> GPLGSPEFENKIEDIGQGAEIIKRTQDITSKRLAICQNIQFDFVKDKKYNKDALVVKMQGFISSRTTYSDLKKYPYIKRMIWPFQYNISLKTKDSNVDLINYLPKNKIDSADVSQKLGYNIGGNFQSAPSIGGSGSFNYSKTISYNQKNYVTEVESQNSKGVKWGVKANSFVTPNGQVSAYDQYLFAQDPTGPA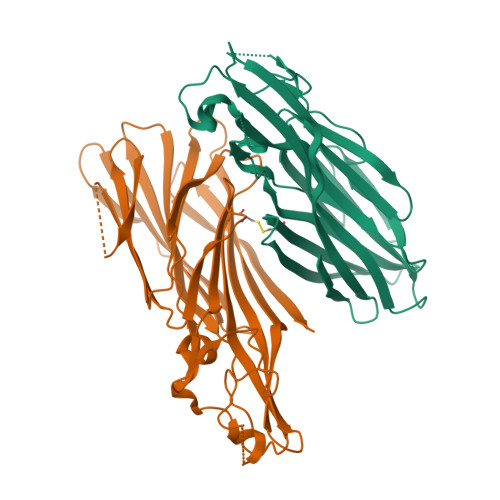ARDYFVPDNQLPPLIQSGFNPSFITTLSHEKGKGDKSEFEITYGRNMDATYAYVTRHRLAVDRKHDAFKNRNVTVKYEVNWKTHEVKIKSITPK;> GPLGSPEFEGKITPVSVKKVDDKVTLYKTTATADSDKFKISQILTFNFIKDKSYDKDTLVLKAAGNINSGYEKPNPNDYDFSKLYWGAKYNVSISSQSNDSVNVVDYAPKNQNEEFQVQNTLGYTFGGDISISNGLSGGLNGNTAFSETINYKQESYRTTLSRCTNYKNVGWGVEAHKIMNNGWGPYGRDSFHPTYGNELFLAGRQSSAYAGQNFIAQHQMPLLSRSNFNPEFLSVLSHRQDGAKKSKITVTYQREMDLYQIRWNGFYWAGANYKNFKTRTFKSTYEIDWENHKVKLLDTKETENNK morpholin-4-yl(1,2,3-thiadiazol-4-yl)methanone | C7 H9 N3 O2 S | 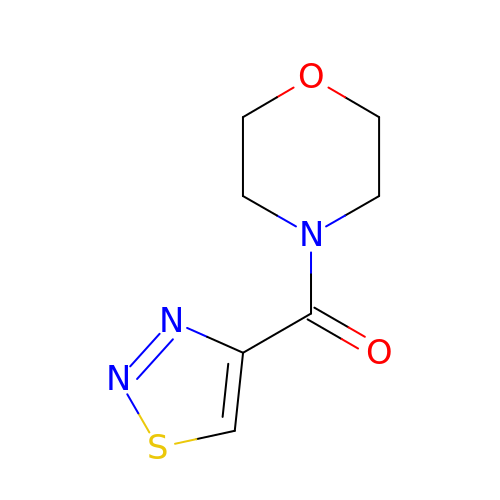BPUDGPLMUNVDOA-UHFFFAOYSA-N> GPGSMADSPVLLVDTTDRVRTLTLNRPQSRNALSAELRSTFFRALSDAQNDDDVDVVIVTGADPVFCAGLDLKELGDTTELPDISPKWPDMTKPVIGAINGAAVTGGLELALYCDILIASENAKFADTHARVGLMPTWGLSVRLPQKVGVGLARRMSLTGDYLSAQDALRAGLVTEVVAHDDLLTAARRVAASIVGNNQKAVRALLDSYHRIDALQTGGALWAEAEAARQWMRSTSGDDIAASRASVIERGRS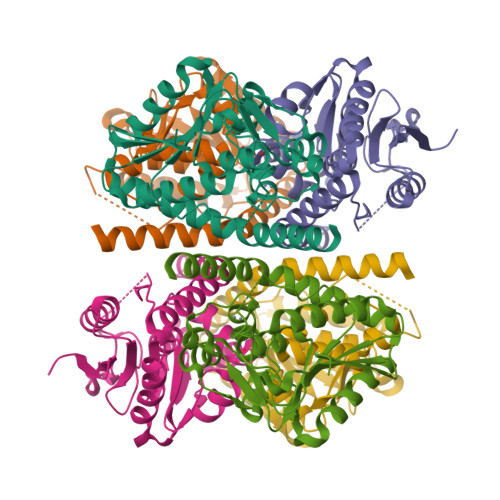QVR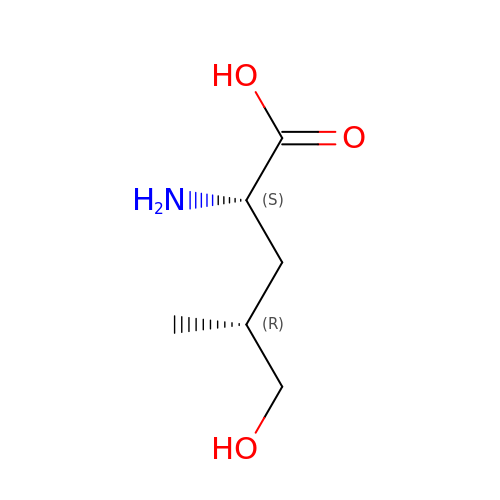(2S,4R)-5-hydroxyleucine | C6 H13 N O3 | SDCAQJCTUOFAKD-UHNVWZDZSA-N>[2x]MALDGIRMPDGCYADGTWELSVHVTDLNRDVTLRVTGEVHIGGVMLKLVEKLDVKKDWSDHALWWEKKRTWLLKTHWTLDKCGIQADAKLQFTPQHKLLRLQLPNMKYVKVKVNFSDRVFKAVSDICKTFNIRHPEELSLLKKPRDPTKKKKKKLDDQSEDEALELEGPLIMPGSGSIYSSPGLYSKTMTPTYDAHDGSPLSPTSAWFGDSALSEGNPGILAVSQPVTSPEILAKMFKPQALLDKAKTNQ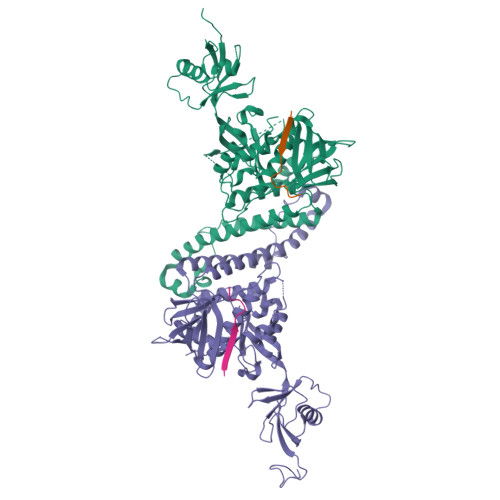GWLDSSRSLMEQDVKENEALLLRFKYYSFFDLNPKYDAIRINQLYEQAKWALLLEEIECTEEEMMMFAALQYHINKLSIMTSENHLTTDVNPECLVSPRYLKKYKSKQITARILEAHQNVAQMSLIEAKMRFIQAWQSLPEFGITHFIARFQGGKREELIGIAYNRLIRMDASTGDAIKTWRFSNMKQWNVNWEIKMVTVEFADEVRLSFICTEVDCKVVHEFIGGYIFLSTRAKDQNESLDEEMFYKLTSGWV;>KSAVTTVVNPQYEGK[2x]>[9x]GSHMSVSFRDRVLKLYLLGFDPSE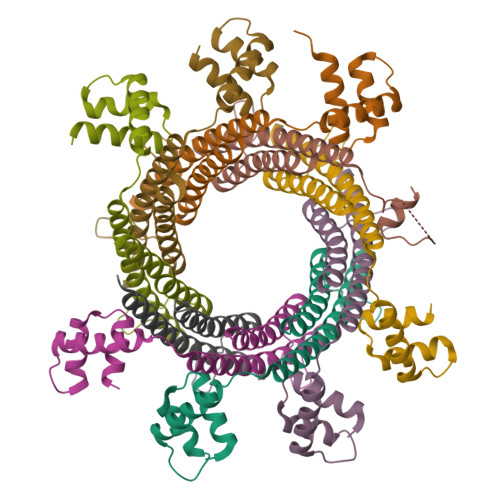IAQTLSLDVKRKVTEEEVLHVLAEARELLSALPSLEDIRAEVGQALERARIFQKDLLAIYQNMLRNYNAMMEGLTEHPDGTPVIGVRPADIAAMADRIMKIDQERITALLNSLKVLG> LRVQFKRMKAAEWARSDVILLESEIGFETDTGFARAGDGHNRFSDLGYISPLDYNLLTNKPNIDGLATKVETAQKLQQKADKETVYTKAESKQELDKKLNLKGGVMTGQLKFKPAATVAYSSSTGGAVNIDLSSTRGAGVVVYSDNDTSDGPLMSLRTGKETFNQSALFVDYKGTTNAVNIAMRQPTTPNFSSALNITSGNENGSAMQLRGSEKALGTLKITHENPSIGADYDKNAAALSIDIVKKTNGAGTAAQGIYINSTSGTTGKLLRIRNLSDDKF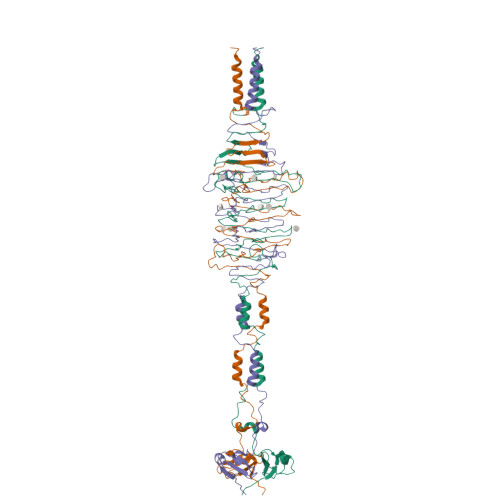YVKSDGGFYAKETSQIDGNLKLKDPTANDHAATKAYVDKAISELKKLILKKH4-[(4-{5-[(3aS,4S,6aR)-2-oxohexahydro-1H-thieno[3,4-d]imidazol-4-yl]pentyl}-1H-1,2,3-triazol-1-yl)methyl]benzoic acid | C20 H25 N5 O3 S | 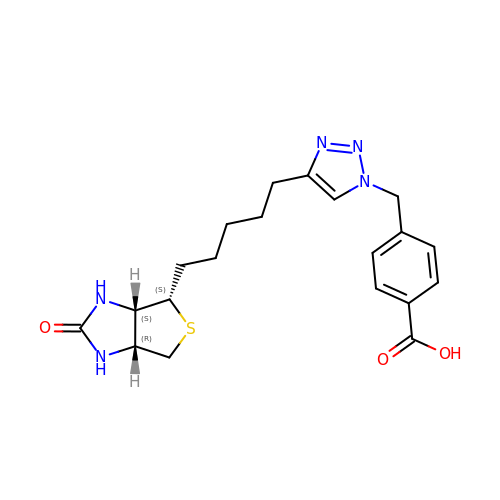WFMFNVSBAHDHPE-BZSNNMDCSA-N>[4x]MVKKPSLAGRLKIIEIDGRKTLGDQHGNPIQLRGMSTHGLQWFPQIINNNAFSALSKDWEANVIRLAMYVGEGGYSTDPSVKEKVIEGINLAIKNDMYVIVDWHI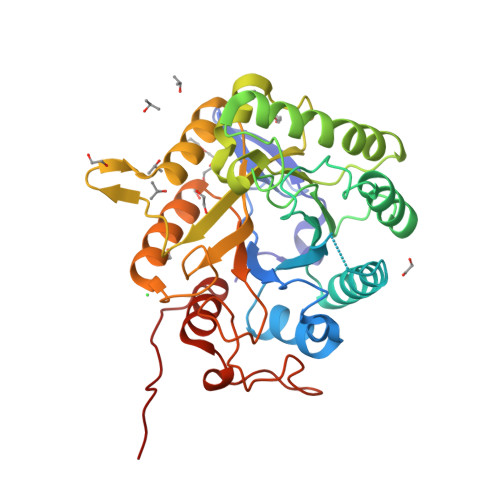LNPGDPNAKIYSGAKEFFKEIASKYPNDLHIIYELANEPNPTESDITNDIAGWEKVKKYAEPIIKMLRDMGNENIIIVGNPEWSTRPDLAVNDPIDDKNVMYSAHFYTGSASVWENGNKGHIARNIEKALENGLTVFVTEWGTSEASGDGGPYLNEADEWLEFLNSNNISWVNWSLANKNEASAAFLPTTSLDPGNGKVWAVNQLSLSGEYVRARIKGIPYKPISRETM>MAAPVVAPPGVVVSRANKRSGAGPGGSGGGGARGAEEEPPPPLQAVLVADSFDRRFFPISKDQPRVLLPLANVALIDYTLEFLTATGVQETFVFCCWKAAQIKEHLLKSKWCRPTSLNVVRIITSELYRSLGDVLRDVDAKALVRSDFLLVYGDVISNINITRALEEHRLRRKLEKNVSVMTMIFKESSPSHPTRCHEDNVVVAVDSTTNRVLHFQKTQGLRRFAFPLSLFQGSSDGVEVRYDLLDCHI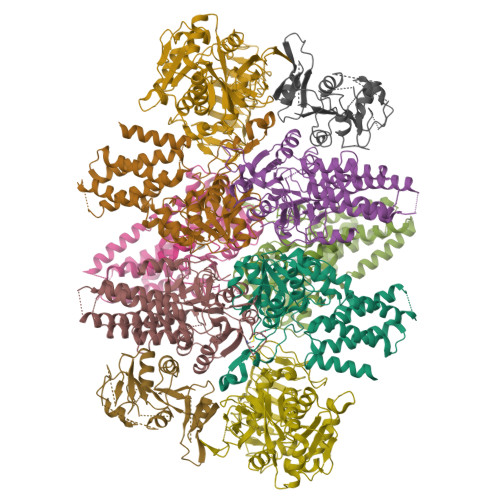SICSPQVAQLFTDNFDYQTRDDFVRGLLVNEEILGNQIHMHVTAKEYGARVSNLHMYSAVCADVIRRWVYPLTPEANFTDSTTQSCTHSRHNIYRGPEVSLGHGSILEENVLLGSGTVIGSNCFITNSVIGPGCHIGDNVVLDQTYLWQGVRVAAGAQIHQSLLCDNAEVKERVTLKPRSVLTSQVVVGPNITLPEGSVISLHPPDAEEDEDDGEFSDDSGADQEKDKVKMKGYNPAEVGAAGKGYLWKAAGMNMEEEEELQQNLWGLKINMEEESESESEQSMDSEEPDSRGGSPQMDDIKVFQNEVLGTLQRGKEENISCDNLVLEINSLKYAYNISLKEVMQVLSHVVLEFPLQQMDSPLDSSRYCALLLPLLKAWSPVFRNYIKRAADHLEALAAIEDFFLEHEALGISMAKVLMAFYQLEILAEETILSWFSQRDTTDKGQQLRKNQQLQRFIQWLKEAEEESSEDD[2x];>[2x]MDYKDDDDKENLYFQSMPGSAAKGSELSERIESFVETLKRGGGPRSSEEMARETLGLLRQIITDHRWSNAGELMELIRREGRRMTAAQPSETTVGNMVRRVLKIIREEYGRLHGRSDESDQQESLHKLLTSGGLNEDFSFHYAQLQSNIIEAINELLVELEGTMENIAAQALEHIHSNEVIMTIGFSRTVEAFLKEAARKRKFHVIVAECAPFCQGHEMAVNLSKAGIETTVMTDAAIFAVMSRVNKVIIGTKTILANGALRAVTGTHTLALAAKHHSTPLIVCAPMFKLSPQFPNEEDSFHKFVAPEEVLPFTEGDILEKVSVHCPVFDYVPPELITLFISNIGGNAPSYIYRLMSELYHPDDHVL;>MAAVAVAVREDSGSGMKAELPPGPGAVGREMTKEEKLQLRKEKKQQKKKRKEEKGAEPETGSAVSAAQCQVGPTRELPESGIQLGTPREKVPAGRSKAELRAERRAKQEAERALKQARKGEQGGPPPKASPSTAGETPSGVKRLPEYPQVDDLLLRRLVKKPERQQVPTRKDYGSKVSLFSHLPQYSRQNSLTQFMSIPSSVIHPAMVRLGLQYSQGLVSGSNARCIALLRALQQVIQDYTTPPNEELSRDLVNKLKPYMSFLTQCRPLSASMHNAIKFLNKEITSVGSSKREEEAKSELRAAIDRYVQEKIVLAAQAISRFAYQKISNGDVILVYGCSSLVSRILQEAWTEGRRFRVVVVDSRPWLEGRHTLRSLVHAGVPASYLLIPAASYVLPEVSKVLLGAHALLANGSVMSRVGTAQLALVARAHNVPVLVCCETYKFCERVQTDAFVSNELDDPDDLQCKRGEHVALANWQNHASLRLLNLVYDVTPPELVDLVITELGMIPCSSVPVVLRVKSSDQ[2x];>[2x]MDDKELIEYFKSQMKEDPDMASAVAAIRTLLEFLKRDKGETIQGLRANLTSAIETLCGVDSSVAVSSGGELFLRFISLASLEYSDYSKCKKIMIERGELFLRRISLSRNKIADLCHTFIKDGATILTHAYSRVVLRVLEAAVAAKKRFSVYVTESQPDLSGKKMAKALCHLNVPVTVVLDAAVGYIMEKADLVIVGAEGVVENGGIINKIGTNQMAVCAKAQNKPFYVVAESFKFVRLFPLNQQDVPDKFKYKADTLKVAQTGQDLKEEHPWVDYTAPSLITLLFTDLGVLTPSAVSDELIKLYLGGENLYFQAEDKGGGSGGGGSGGGGSASQGGLNDIFEAQKIEWHEGGGGSGGGGSGGGGSGRDQDYKDDDDK;>[2x]MEFQAVVMAVGGGSRMTDLTSSIPKPLLPVGNKPLIWYPLNLLERVGFEEVIVVTTRDVQKALCAEFKMKMKPDIVCIPDDADMGTADSLRYIYPKLKTDVLVLSCDLITDVALHEVVDLFRAYDASLAMLMRKGQDSIEPVPGQKGKKKAVEQRDFIGVDSTGKRLLFMANEADLDEELVIKGSILQKHPRIRFHTGLVDAHLYCLKKYIVDFLMENGSITSIRSELIPYLVRKQFSSASSQQGQEEKEEDLKKKELKSLDIYSFIKEANTLNLAPYDACWNACRGDRWEDLSRSQVRCYVHIMKEGLCSRVSTLGLYMEANRQVPKLLSALCPEEPPVHSSAQIVSKHLVGVDSLIGPETQIGEKSSIKRSVIGSSCLIKDRVTITNCLLMNSVTVEEGSNIQGSVICNNAVIEKGADIKDCLIGSGQRIEAKAKRVNEVIVGNDQLMEI>[3x]MNAIKLYPLKKLEIILEGAHKEFATD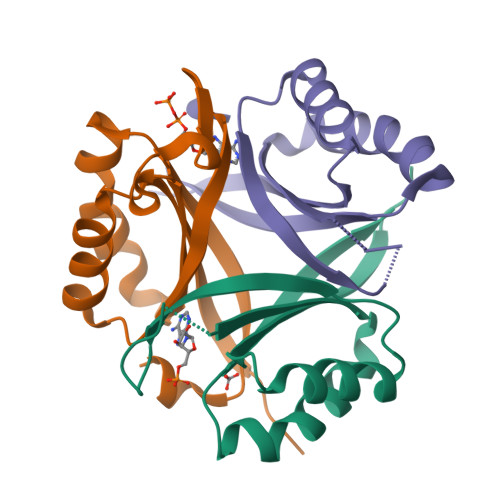LLDRAGVKGYTIVGNLSGKGSHGMYEGHLMFNEDDALIMIIAAVPEELVGPLLEGFQPFFEAHSGVVFVHDIQVGRPIKFRN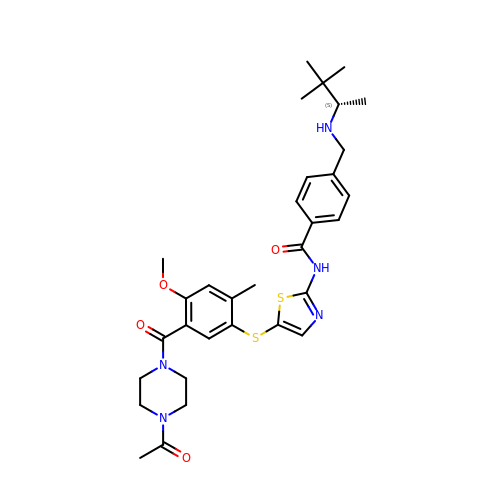N-[5-({5-[(4-acetylpiperazin-1-yl)carbonyl]-4-methoxy-2-methylphenyl}sulfanyl)-1,3-thiazol-2-yl]-4-({[(1S)-1,2,2-trimethylpropyl]amino}methyl)benzamide | C32 H41 N5 O4 S2 | ZHXNIYGJAOPMSO-NRFANRHFSA-N> DVSFRLSGADPRSYGMFIKDLRNALPFREKVYNIPLLLPSVSGAGRYLLMHLFNYDGKTITVAVDVTNVYIMGYLADTTSYFFNEPAAELASQYVFRDARRKITLPYSGNYERLQIAAGKPREKIPIGLPALDSAISTLLHYDSTAAAGALLVLIQTTAEAARFKYIEQQIQERAYRDEVPSLATISLENSWSGL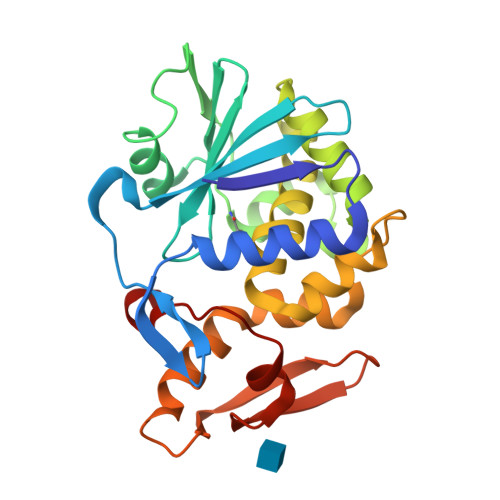SKQIQLAQGNNGIFRTPIVLVDNKGNRVQITNVTSKVVTSNIQLLLNTRNI> MSQQVDKIKASYPLFLDQDYKDMLAKKRDGFEEKYPQDKIDEVFQWTTTKEYQELNFQREALTVNPAKACQPLGAVLCALGFEKTMPYVHGSQGCVAYFRSYFNRHFREPVSCVSDSMTEDAAVFGGQQNMKDGLQNCKATYKPDMIAVSTTCMAEVIGDDLNAFINNSKKEGFIPDEFPVPFAHTPAFVGSHVTGWDNMFEGIARYFTLKSMDDKVVGSNKKINIVPGFETY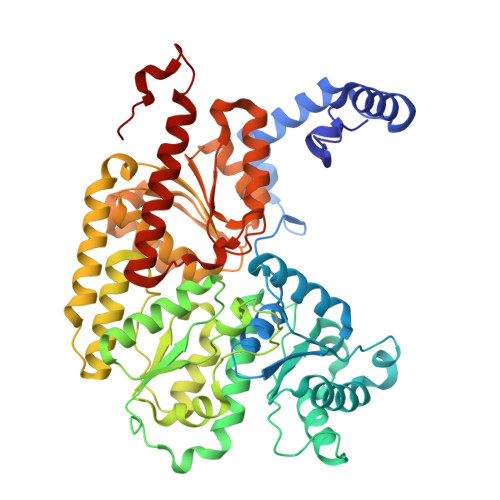LGNFRVIKRMLSEMGVGYSLLSDPEEVLDTPADGQFRMYAGGTTQEEMKDAPNALNTVLLQPWHLEKTKKFVEGTWKHEVPKLNIPMGLDWTDEFLMKVSEISGQPIPASLTKERGRLVDMMTDSHTWLHGKRFALWGDPDFVMGLVKFLLELGCEPVHILCHNGNKRWKKAVDAILAASPYGKNATVYIGKDLWHLRSLVFTDKPDFMIGNSYGKFIQRDTLHKGKEFEVPLIRIGFPIFDRHHLHRSTTLGYEGAMQILTTLVNSILERLDEETRGMQATDYNHDLVR> MMASTALSLMGRCNPDGCTRGKHVTAAPMDGPRGPSSLAGTFGWGLAIPAGEPCGRVCSPATVGFFPVAKKSNKENRPEASGLPLESERTGDNPTVRGSAGADPVGQDAPGWTCQFCERTFSTNRGLGVHKRRAHPVETNTDAAPMMVKRRWHGEEIDLLARTEARLLAERGQCSGGDLFGALPGFGRTLEAIKGQRRREPYRALVQAHLARFGSQPGPSSGGCSAEPDFRRASGAEEAGEERCAEDAAAYDPSAVGQMSPDAARVLSELLEGAGRRRACRAMRPKTAGRRNDLHDDRTASAHKTSRQKRRAEYARVQELYKKCRSRAAAEVIDGACGGVGHSLEEMETYWRPILERVSDAPGPTPEALHALGRAEWHGGNRDYTQLWKPISVEEIKASRFDWRTSPGPDGIRSGQWRAVPVHLKAEMFNAWMARGEIPEILRQCRTVFVPKVERPGGPGEYRPISIASIPLRHFHSILARRLLACCPPDARQRGFICADGTLENSAVLDAVLGDSRKKLRECHVAVLDFAKAFDTVSHEALVELLRLRGMPEQFCGYIAHLYDTASTTLAVNNEMSSPVKVGRGVRQGDPLSPILFNVVMDLILASLPERVGYRLEMELVSALAYADDLVLLAGSKVGMQESISAVDCVGRQMGLRLNCRKSAVLSMIPDGHRKKHHYLTERTFNIGGKPLRQVSCVERWRYLGVDFEASGCVTLEHSISSALNNISRAPLKPQQRLEILRAHLIPRFQHGFVLGNISDDRLRMLDVQIRKAVGQWLRLPADVPKAYYHAAVQDGGLAIPSVRATIPDLIVRRFGGLDSSPWSVARAAAKSDKIRKKLRWAWKQLRRFSRVDSTTQRPSVRLFWREHLHASVDGRELRESTRTPTSTKWIRERCAQITGRDFVQFVHTHINALPSRIRGSRGRRGGGESSLTCRAGCKVRETTAHILQQCHRTHGGRILRHNKIVSFVAKAMEENKWTVELEPRLRTSVGLRKPDIIASRDGVGVIVDVQVVSGQRSLDELHREKRNKYGNHGELVELVAGRLGLPKAECVRATSCTISWRGVWSLTSYKELRSIIGLREPTLQIVPILALRGSHMNWTRFNQMTSVMGGGVG

Pioneering research on the Bombyx mori (silk moth) R2 element (R2Bm), which selectively inserts into the 28S rRNA gene, has contributed significantly to our understanding of this type of MGE. R2, like all non-LTR retrotransposons, encodes an open reading frame (ORF) with DNA-binding, endonuclease, and reverse transcriptase activities. The endonuclease domain (restriction-like endonuclease, RLE) nicks the target DNA, and the reverse transcriptase domain uses the exposed 3’ end from the nick to prime reverse transcription of the R2 RNA, resulting in a new genomic copy of the R2 element. To address these questions, we solved a cryo-EM structure of the Bombyx mori R2 protein (R2Bm) initiating TPRT at the 28S rRNA gene using its own 3′UTR.

To assemble a complex stalled during initiation of TPRT, we incubated R2Bm with target DNA, 3′UTR RNA, and the chain-terminator nucleotide 2′,3′-dideoxythymidine (ddT), which mimics the first nucleotide incorporated in the TPRT reaction (dT) but does not allow further elongation. To overcome these issues, we used a carbon support on the cryo-EM grid and added 5 nt of downstream 28S RNA sequence to the 3′ end of the 3′UTR RNA to stabilize the complex by forming a primer-template duplex with the target DNA bottom strand. The two strands of the target DNA separate around the ZnF domain, with the bottom strand feeding into the RLE active site where the scissile phosphate remains bound, while the top strand snakes along the opposing surface of the RLE. The RT active site contains a heteroduplex formed by the nicked bottom strand of the target DNA (5′ to the cleavage site) and the 5 nt of 28S RNA homology extension beyond the 3′UTR RNA. This target heteroduplex is surrounded by residues important for RT activity, and the cryo-EM density shows incorporation of the ddT chain terminator nucleotide into the bottom strand. The 248-nt 3′UTR RNA is mostly not resolved in the cryo-EM density except for a core 40-nt region, which wraps around the NTE-1 ɑ helix of R2Bm and the 3′ end of which is guided into the RT active site via the NTE0 domain. Based on the structure, however, we predicted that two regions are key for sequence-specific DNA recognition by R2Bm: a 13-bp upstream motif from –34 to –22, which is bound by the N-terminal N-ZnF and Myb domains, and the 7 bp from –6 to +1, which are bound by the RLE. We term these regions the Retrotransposon Upstream Motif (RUM) and Retrotransposon-Associated INsertion site (RASIN), respectively. In our structure, the 11 base pairs of the RASIN from –6 to +5 are melted around the RLE domain. P1 and J1/2 are mainly recognized by an ɑ helix from the R2Bm NTE-1 domain, which packs into the major groove of P1 and is wrapped by J1/2.4-[4-[[7-(dimethylamino)-2,1,3-benzoxadiazol-4-yl]sulfonyl]piperazin-1-yl]sulfonyl-5-pyridin-3-yl-benzene-1,2-diol 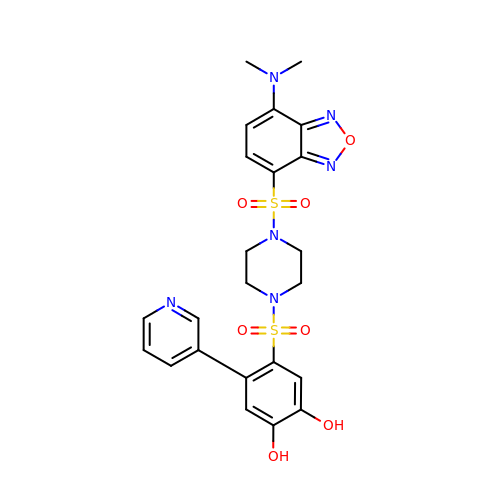| C23 H24 N6 O7 S2 | DEHSUWFLXFTDPH-UHFFFAOYSA-N>MASMTGGQQMGRGSAEAG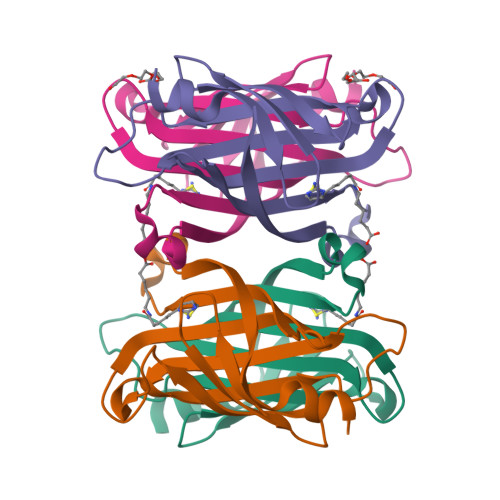ITGTWSDQLGDTFIVTAGADGALTGTYENAVGNAESRYVLTGRYDSAPATDGSGTALGWTVAWKNNSKNAHSATTWSGQYVGGADAKINTQWLLTSGTTNANAWKSTLVGHDTFTKVKPSAASHHHHHH[4x]> MAHHHHHHMITERELLDYIVNNGGFLD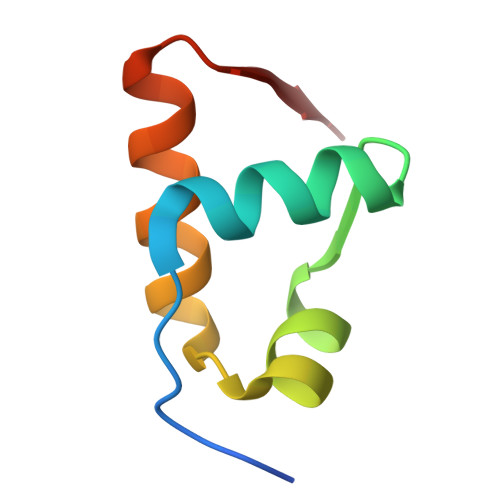IEHFSKVYGVEKQEVVKLLEALKNKGLIAVES> GSHMSLDNKPIMRVASIDIGSYSVRLTIAQIKDGKLSIILERGRITSLGTKVKETGRLQEDRIEETIQVLKEYKKLIDEFKVERVKAVATEAIRRAKNAEEFLERVKREVGLVVEVITPEQEGRYAYLAVAYSLKPEGEVCVVDQGGGSTEYVFGKGYKVREVISLPIGIVNLTETFFKQDPPTEEEVKRFFEFLEKELSKVKKPVDTIV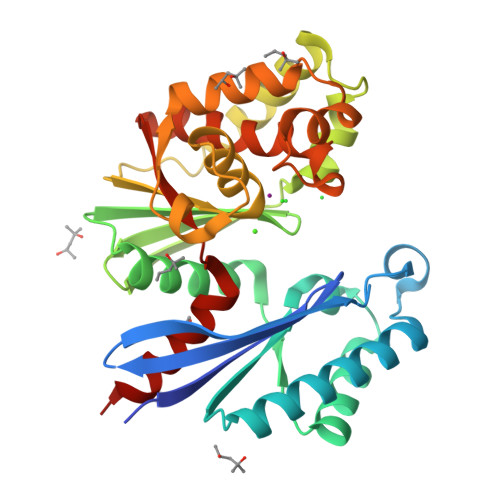GLGGTITTLAALEYNVYPYDPQKVHGKVLTYGQIKKWFDTFKEIPSEERSKRFRQVEDRRAKVILAGIGIFLKTLEIFEKDCLIVSDWGLREGVLVSEVLKENHS>[4x]MMIFFLSLSLESCSKEDDNNPSNSENNGGNNNLGTELDYDTFCFYYDWY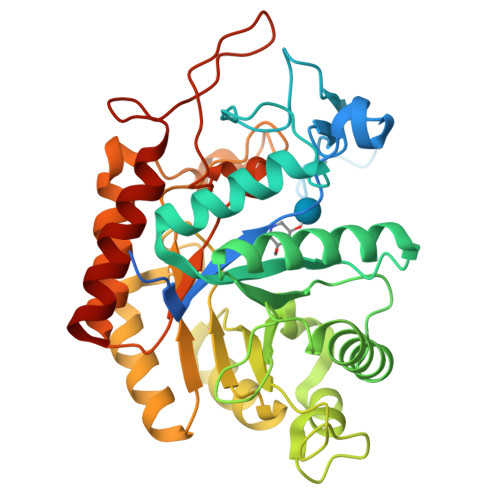GSEAIDGQYRHWAHAIAPDPNGGSGQNPGTIPGTQESIASNFYPQLGRYSSSDPNILTKHMDMFVMARTGVLALTWWNEQDETEAKRIGLILDAADKKKIKVCFHLEPYPSRNVQNLRENIVKLITRYGNHPAFYRKDGKPLFFIYDSYLIEPSEWEKLLSPGGSITIRNTAYDALMIGLWTSSPTVQRPFILNAHFDGFYTYFAATGFTYGSTPTNWVSMQKWAKENGKIFIPSVGPGYIDTRIRPWNGSVIRTRTDGQYYDAMYRKAIEAGVSAISITSFNEWHEGSQIEPAVPYTSSEFTYLDYENREPDYYLTRTAYWVGKFRESKQ>[7x]MALKTKPRWDKYDGYVGNYRGVLGEDIDLDTEANRVLAVGTNSNGAIVVGAGQTGIKGLMIVAVGADIHGAMLDGGINNHAGDPQDVGKHGEITNFQPTVFGRTFGVAISATEGNVKLAVNGVDTGNIAYDTSAANLKSGIVAVDDGFTADDFTVTGTAPNFTIVTTRTDVTITASGEGVTVTEATSVAAAGTNYYGHADGTVNAVKGSDGVYVGHTQEADRLIVNVKDEED;>[7x]MA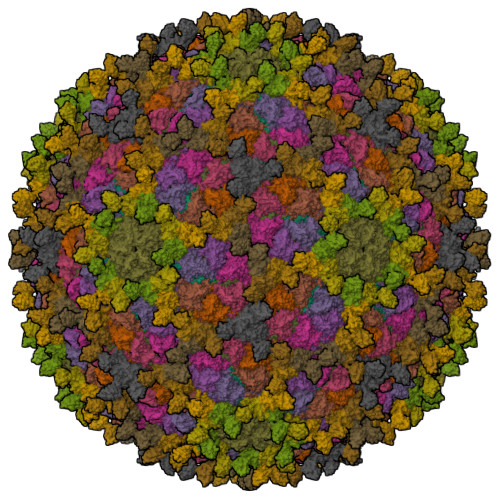TKELKIGGVPVFPIFGGTAPVRQEGIMTQGDLVTVTSDGIDLNALWNSFAESIAIYNEAMDNLIQLLTYPVTVPVEPVVQIGETTFEEATELGVPRGAGLPIEVFQMGYDLRHYDKRNAYSWMFLADADGRQVEAIHDAVLWADKRLVFRKVMEALFDNRTRRANIRNQAYNVYPLYNGDGVPPPRFKNNVFDETHSHYVISHNSVVDSSDLEDLMELLAEHGYSPQAGTQFLLLANKAETDAIRQFRRGVVNNNGATAGYDFIPSPTQPAMMLPNAEGLLGNQPAPTFGGLAVIGSYGFWNIVEEDYIPPGYLVGVGYGGAFNLGNPVGLRQHANPAMQGLRIIAGNYQRYPLVDGFYARSFGTGVRQRGGAAIMQIKASGAYECPPIYKKGGGFLV;>MANRTVSPSTQGVRPAMRQMYNGRNVATRPIPLIVDTSEIRAIMAAAADARPKTSAVNFPQSGPRPAGAAVVFGTKVSGAPGNVVSNNAATFAPLTGTQNFE[2x]> FDCGKPQVEPKKCPGRVVGGCVAHPHSWPWQVSLRTRFGMHFCGGTLISPEWVLTAAHCLEKSPRPSSYKVILGAHQEVNLEPHVQEIEVSRLFLEPTRKDIALLKLSSPAVITDKVIPACLPSPNYVVADRTECFITGWGETQGTFGAGLLKEAQLPVIENKVCNRYEFLNGRVQ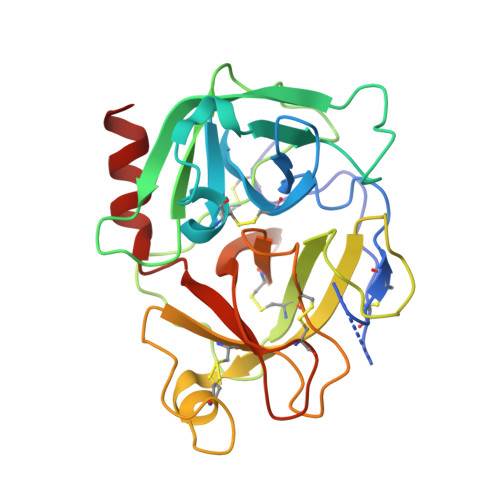STELCAGHLAGGTDSCQGDAGGPLVCFEKDKYILQGVTSWGLGCARPNKPGVYVRVSRFVTWIEGVMRNN> RVCGVSAARLTPCGTGTSTDVVYRAFDIYNDKVAGFAKFLKTNCCRFQEKDEDDNLIDSYFVVKRHTFSNYQHEETIYNLLKDCPAVAKHDFFKFRIDGDMVPHISRQRLTKYTMADLVYALRHFDEGNCDTLKEILVTYNCCDDDYFNKKDWYDFVENPDILRVYANLGERVRQALLKTVQFCDAMRNAGIVGVLTLDNQDLNGNWYDFGDFIQTTPGSGVPVVDSYYSLLMPILTLTRALTAESHVDTDLTKPYIKWDLLKYDFTEERLKLFDRYFKYWDQTYHPNCVNCLDDRCILHCANFNVLFSTVFPPTSFGPLVRKIFVDGVPFVVSTGYHFRELGVVHNQDVNLHSSRLSFKELLVYAADPAMHAASGNLLLDKRTTCFSVAALTNNVAFQTVKPGNFNKDFYDFAVSKGFFKEGSSVELKHFFFAQDGNAAISDYDYYRYNLPTMCDIRQLLFVVEVVDKYFDCYDGGCINANQVIVNNLDKSAGFPFNKWGKARLYYDSMSYEDQDALFAYTKRNVIPTITQMNLKYAISAKNRARTVAGVSICSTMTNRQFHQKLLKSIAATRGATVVIGTSKFYGGWHNMLKTVYSDVENPHLMGWDYPKCDRAMPNMLRIMASLVLARKHTTCCSLSHRFYRLANECAQVLSEMVMCGGSLYVKPGGTSSGDATTAYANSVFNICQAVTANVNALLSTDGNKIADKYVRNLQHRLYECLYRNRDVDTDFVNEFYAYLRKHFSMMILSDDAVVCFNSTYASQGLV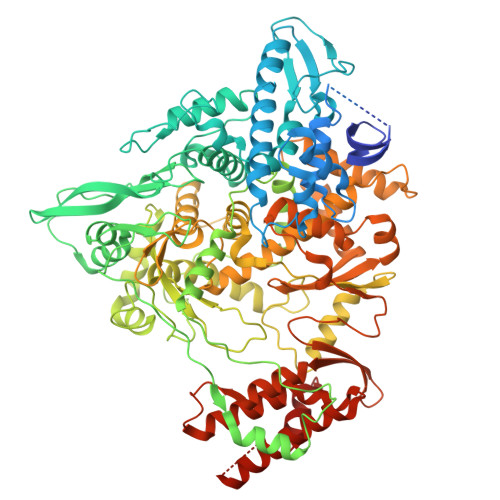ASIKNFKSVLYYQNNVFMSEAKCWTETDLTKGPHEFCSQHTMLVKQGDDYVYLPYPDPSRILGAGCFVDDIVKTDGTLMIERFVSLAIDAYPLTKHPNQEYADVFHLYLQYIRKLHDELTGHMLDMYSVMLTNDNTSRYWEPEFYEAMYTPHTVLQ> MLG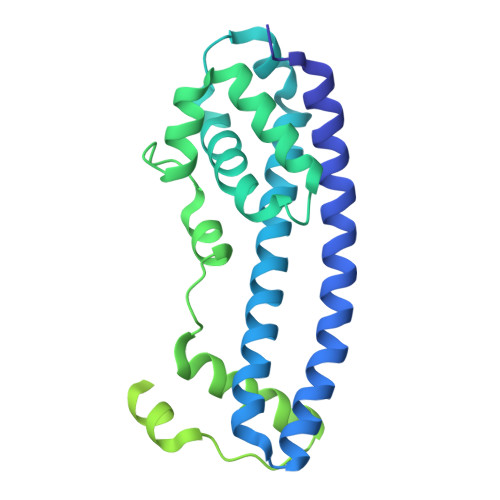SGFKAERLRVNLRLVINRLKLLEKKKTELAQKARKEIADYLAAGKDERARIRVEHIIREDYLVEAMEILELYCDLLLARFGLIQSMKELDSGLAESVSTLIWAAPRLQSEVAELKIVADQLCAKYSKEYGKLCRTNQIGTVNDRLMHKLSVEAPPKILVERYLIEIAKNYNVPYEPDSVVMAEAPPGVETDLIDVGFTDDVKKGGPGRGGSGGFTAPVGGPDGTVPMPMPMPMPSANTPFSYPLPKGPSDFNGLPMGTYQAFPNIHPPQIPATPPSYESVDDINADKNISSAQIVGPGPKPEASAKLPSRPADNYDNFVLPELPSVPDTLPTASAGASTSASEDIDFDDLSRRFEELKKKT(2S)-2-hydroxy-2-(oxan-4-yl)acetamide | C7 H13 N O3 | 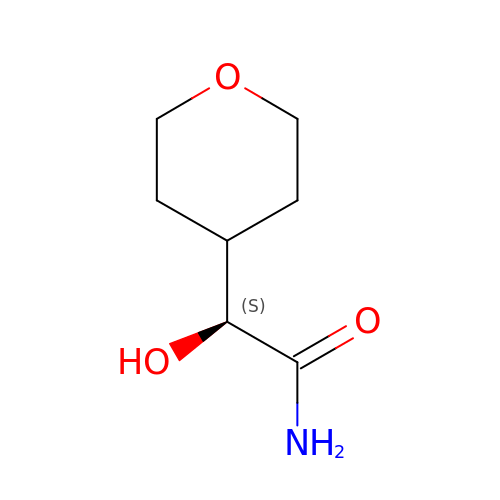KOEHHYFUIVEIQO-UHFFFAOYSA-N>MGSDKIHHHHHHENLYFQGMFITTEGINAGYTIKDVVEATSSLMLASEDIDKYNMFDQLFDEAKQKLKKKADLL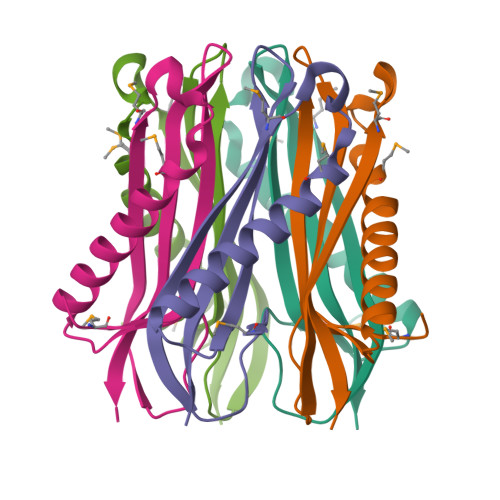EGDGIIGLKYNTEVVEVNGAPKFLVVHGYGTVILIDK[5x]>[72x]MGLFDRIKRVVSSNLNDLVNKAEDPEKMLEQAILEMQEDLVQLRQGVAQAIAAQKRSEKQYNDAQNEINKWQRNAQLALQKGDENLARQALERKKTYTDTSAALKASLDTQSTQVETLKRNLIQLESKISEAKTKKEMLKARITTAKAQEQLQGMVRGMNTSSAMSAFERMEEKVLMQESRAQALGELAGADLETQFAQLEGGSDVDDELAALKAQMLPPATPVTQAQLPPQQETTPAKSNEVVDAELDSLRKQLDQL

Proteins that perform these functions include Vipp1/IM30 in photosynthetic plastids, PspA in bacteria, and ESCRT-III in eukaryotes. Here, using a combination of evolutionary and structural analyses, we show that these protein families are homologous and share a common ancient evolutionary origin that likely predates the last universal common ancestor. This homology is evident in cryo-electron microscopy structures of Vipp1 rings from the cyanobacterium Nostoc punctiforme presented over a range of symmetries. Rings have an inner lumen that is able to bind and deform membranes.

Reconstructions were also generated for the other six symmetries and complete ring models built. Rungs are maximally constricted at the top and bottom with internal lumen diameters of 14 nm and 15.7 nm, and widest at the ring equator between rungs 3 and 4 with an internal diameter of 17.5 nm. This unique asymmetric curvature is a feature of all Vipp1C11–C17 ring symmetries. The analysis of different ring symmetries, ranging from C11–C17, provides us with a view of the structural flexibility that enables Vipp1, PspA, and ESCRT-III family members to perform their functions. Furthermore, as each ring comprises between 5–7 rungs stacked together to build a dome-shaped architecture, these asymmetric structures provide us with a glimpse of the structural features that enable filament tilt in the context of an ESCRT-III-like polymer. Based on the Vipp1C11–C17 models, where helix α5C is positioned at the tip of the spike, α6 helices likely coat the ring outside surface and do not contribute directly to polymer formation. Consistent with this, Interfaces 1 and 3 linking the top two rungs were poorly resolved in Vipp1C11–C17 rings, indicating a weak interaction once the limiting geometry is reached. When membrane was modeled into the Vipp1C11–C17 structures as a 4-nm bilayer, sequential constriction was observed with the membrane lumen reaching ∼3 nm within Vipp1C11.>MKIQMRNKKVLSFLTLTAIVSQALVYPVYAQTSTSNHSNKKKEIVNEDILPNNGLMGYYFTDEHFKDLKLMAPIKDGNLKFEEKKVDKLLDKDKSDVKSIRWTGRIIPSKDGEYTLSTDRDDVLMQVNTESTISNTLKVNMKKGKEYKVRIELQDKNLGSIDNLSSPNLYWELDGMKKIIPEENLFLRDYSNIEKDDPFIPNNNFFDPKLMSDWEDEDLDTDNDNIPDSYERNGYTIKDLIAVKWEDSFAEQGYKKYVSNYLESNTAGDPYTDYEKASGSFDKAIKTEARDPLVAAYPIVGVGMEKLIISTNEHASTDQGKTVSRATTNSKTESNTAGVSVNVGYQNGFTANVTTNYSHTTDNSTAVQDSNGESWNTGLSINKGESAYINANVRYYNTGTAPMYKVTPTTNLVLDGDTLSTIKAQENQIGNNLSPGDTYPKKGLSPLALNTMDQFSSRLIPINYDQLKKLDAGKQIKLETTQVSGNFGTKNSSGQIVTEGNSWSDYISQIDSISASIILDTENESYERRVTAKNLQDPEDKTPELTIGEAIEKAFGATKKDGLLYFNDIPIDESCVELIFDDNTANKIKDSLKTLSDKKIYNVKLERGMNILIKTPTYFTNFDDYNNYPSTWSNVNTTNQDGLQGSANKLNGETKIKIPMSELKPYKRYVFSGYSKDPLTSNSIIVKIKAKEEKTD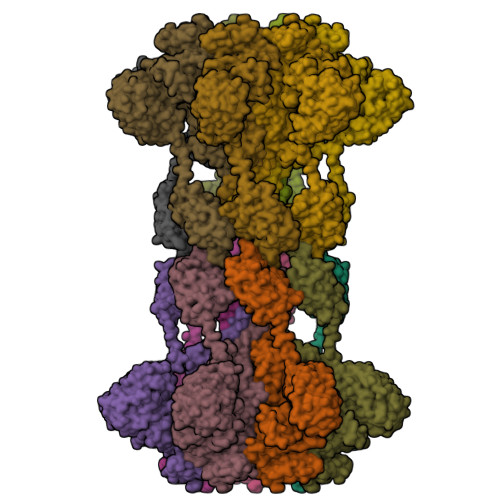YLVPEQGYTKFSYEFETTEKDSSNIEITLIGSGTTYLDNLSITELNSTPEILDEPEVKIPTDQEIMDAHKIYFADLNFNPSTGNTYINGMYFAPTQTNKEALDYIQKYRVEATLQYSGFKDIGTKDKEMRNYLGDPNQPKTNYVNLRSYFTGGENIMTYKKLRIYAITPDDRELLVLSVD[14x]> GHMAPAPPANSGESSLLSESELPAGISYAEAMEGGSRPLLHPDNPVVFFDISIGSHEAGRIKIELFKNLAPKSAENFRQFCTGEFRQNQVPIGYKGATFHRIIKNFMIQGGDFVKGDGTGRLSIYGSSFPDEAFVLPHFRSGLLSLANSGPDTNGCQFFITCAKCDWLNRKHVVFGQ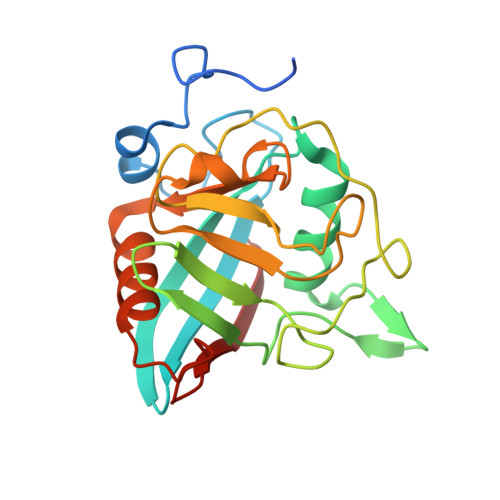VLGKESMQVVRKIEHVTVDGGNRPRIPVTVTQCGEL> MSLHPHAMPDMGPDMNKVPWMGDEQIAMLVYPGMTVMDLVGPHCMFGSLMGAKIYIVAKSLDPVTSDAGLAIVPTATFGTCPRDLTVLFAPGGTDGTLAAASDAETLAFMADRGARAKYITSVCSGSLILGAAGLLKGYKATSHWSCRDALAGFGAIPTEARVVRDRNRITGAGVTAGLDFGLSMVAELRDQTYAECAQLMSEYDPDPPFNAGSMKTAPAHVRTAMIELVAEFTKKADALAGFPKEGHHH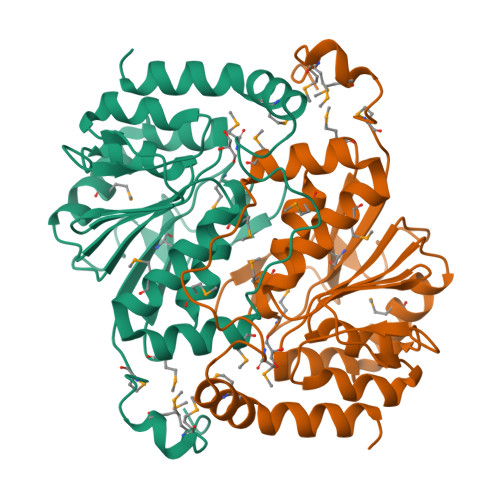HHH>MRR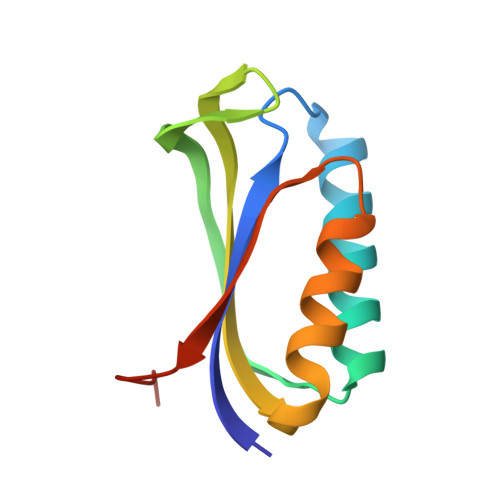YEVNIVLNPNLDQSQLALEKEIIQRALENYGARVEKVAILGLRRLAYPIAKDPQGYFLWYQVEMPEDRVNDLARELRIRDNVRRVMVVKSQEPFLANA[2x]>MSTNKVNKERTFLAVKPDGVARGLVGEIIARYEKKGFVLVGLKQLVPTKDLAESHYAEHKERPFFGGLVSFITSGPVVAMVFEGKGVVASAR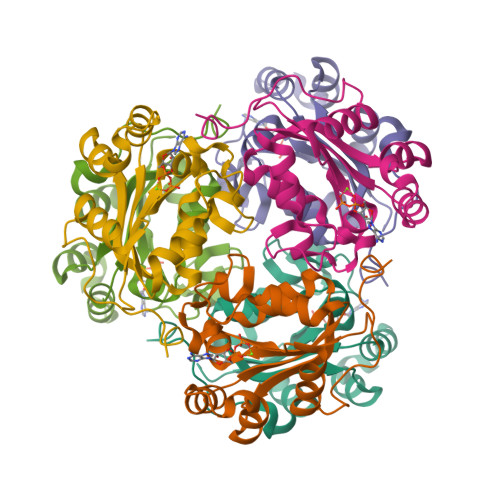LMIGVTNPLASAPGSIRGDFGVDVGRNIIHGSDSVESANREIALWFKPEELLTEVKPNPNLYE[2x]> EDVAKMQEDLESMHPLLEEAAK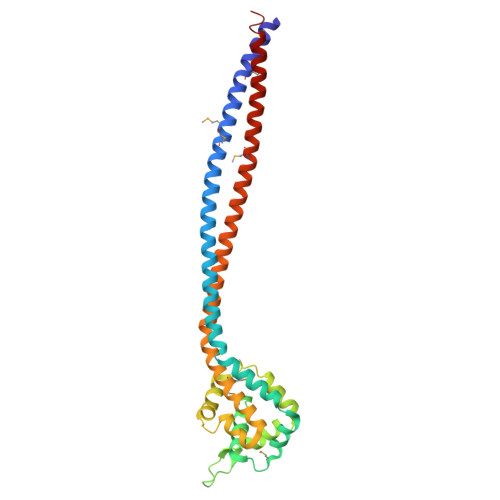DTMLTMEQIKVDTAIAEETRNSVQTEEIKANEKAKKAQAIADDAQKDLDEALPALDAALASLRNLNKNDVTEVRAMQRPPPGVKLVIEAVCIMKGIKPKKVPGEKPGTKVDDYWEPGKGLLQDPGHFLESLFKFDKDNIGDVVIKAIQPYIDNEEFQPATIAKVSKACTSICQWVRAMHKYHFVAKAVEPKRQALLEAQDDLGVTQRILDEAKQRLREVEDGIATMQAKYRECITKKEELELKCEQCEQRLGRAG> E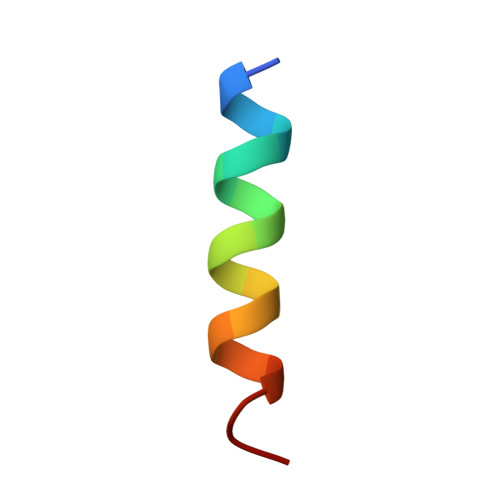QLLKALEFLLKELLEKL Alkane monooxygenase (AlkB) is a widely occurring integral membrane metalloenzyme that catalyzes the initial step in the functionalization of recalcitrant alkanes with high terminal selectivity. AlkB enables diverse microorganisms to use alkanes as their sole carbon and energy source. Alkane monooxygenase (AlkB) is a transmembrane metalloenzyme that catalyzes terminal hydroxylation reactions of alkanes with broad chain-length specificity and exclusive terminal C–H bond selectivity. AlkG, an [Fe–4S] rubredoxin, docks via electrostatic interactions and sequentially transfers electrons to the diiron center.

Here we present the 48.6-kDa cryo‐electron microscopy structure of a natural fusion from Fontimonas thermophila between AlkB and its electron donor AlkG at 2.76 Å resolution. The solved FtAlkBG structure is a monomer, consisting of both AlkB (residues 13–387) and AlkG (residues 415–467) domains, with a total molecular mass of 48.6 kDa. The FtAlkB structure is mostly α-helical, with six transmembrane α-helices (TM1–6), two partially membrane-embedded short α-helices α2 and α3, a long membrane-associated amphiphilic helix α4 and six other α-helices outside the membrane. The diiron center is coordinated by nine conserved histidines and one carboxylate residue with His137, His141, His167, His172 and His314 coordinating Fe1 and four histidines (His171, His272, His311 and His315) and glutamate Glu271 coordinating Fe2. Additional density was present in the active site of the cryo-EM structure, allowing a dodecane substrate (C-12) to be modeled with its terminal methyl group in close proximity of the diiron center. The linear dodecane is oriented by hydrophobic residues, such that its terminal methyl group (C(sp3)–H bonds) is 5.3 Å from Fe1 and 4.8 Å from Fe2. The proximity of the substrate terminal methyl group to Fe2 suggests the Fe2 center may be more directly involved in C–H bond activation. FtAlkBG has a long, hydrophobic substrate binding channel starting from near the middle of transmembrane helices TM1 and TM2 and ending at the diiron center. FtAlkG sits on a positively charged surface of FtAlkB, adjacent to the diiron center. Although there are two irons in FtAlkB, the [Fe–4S] cluster in FtAlkG is closer to Fe1, that is, at 13.6 Å, than to Fe2, at 17.1 Å.

> SNAMSTPTLDAGTLAWNDGKRYLWLLSPFIPVLGLIGLGLFLYTDIGLFTWSGPLLIYGLIPLLDWLVGEDRNNPPEAAVAQLENDRYYRAIVYAYLPTQYAVTVLGTWVAVTADLAIWEYIGLVLSVGAVNGIGINTAHELGHKRENLDRWLAKLTLAPVAYGHFFVEHNRGHHKNVATPEDPASSKMGESFWAFLPRTVIGSLRSAWAIEKARLQRNKQSVWSLDNENLQAWAMTIVLFGALTACLGWPALLFLVLQAAYGASLLEVINYIEHYGLLRQKLPDGRYERCQPRHSWNSNHIVTNLFLYQLQRHSDHHANPTRRFQALRHFDDSPQLPSGYASMLIPAYVPWLWFRLMDPLVARHYGGDLTKANLYPPKRAALLARWHRPRPDARRADTQPTDATATPADAAASPGGRYQCTDCGYIYDEAIGCPREGFPPGTPWSQIPDDWSCPDCAVRDKVDFRKLPAA methyl 5-(6-{[(cis-4-hydroxycyclohexyl)amino]methyl}-2,4-dihydroindeno[1,2-c]pyrazol-3-yl)furan-2-carboxylate 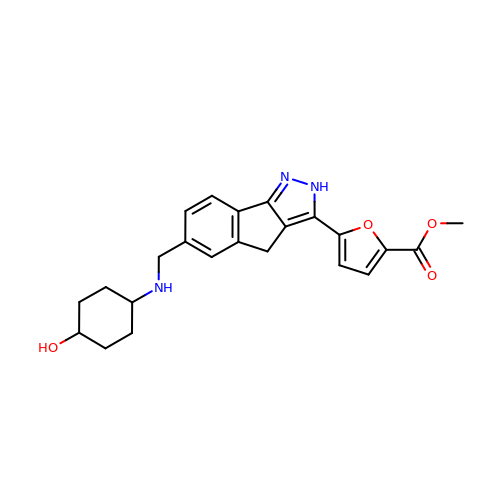| C23 H25 N3 O4 | MCIHIBVPUQANQG-IYBDPMFKSA-N> MSLQGIHLSDLSYKHAILKESQYTIKRDVGTTTAVTPSSLQQEITLLCGEILYAKHADYKYAAEIGIQYISTALGSERVQQILRNSGSEVQVVLTRTYSLG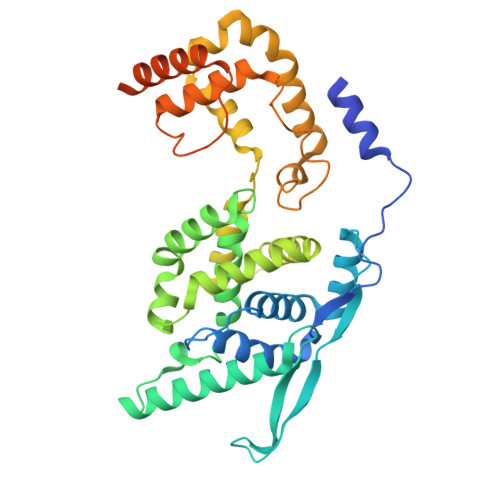KIKNNKGEDLQMLDIHGVEKSWVEEIDKEARKTMATLLKESSGNIPQNQRPSAPDTPIILLCVGALIFTKLASTIEVGLETTVRRANRVLSDALKRYPRMDIPKIARSFYDLFEQKVYHRSLFIEYGKALGSSSTGSKAESLFVNIFMQAYGAGQTMLRWGVIARSSNNIMLGHVSVQAELKQVTEVYDLVREMGPESGLLHLRQSPKAGLLSLANCPNFASVVLGNASGLGIIGMYRGRVPNTELFSAAESYAKSLKESNKINFSSLGLTDEEKEAAEHFLNVSDDSQNDYEKHHHHHH>[4x]MASHGKQFTLYTHNSGPNGWKVAIVLEELGLSYEPVFLDLMKGEHKAPEYLKINPNGRVPALIDHKNNNYTVWESNAVTQYLVDKY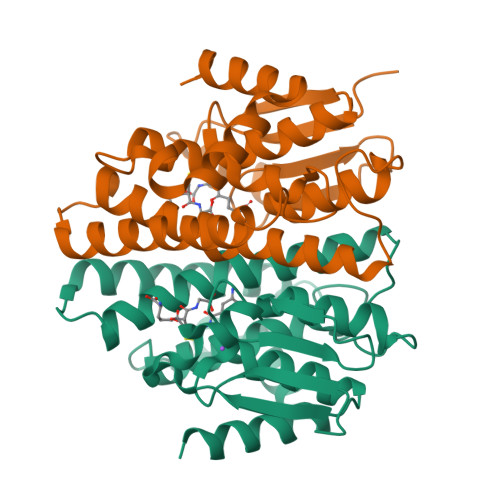DNDRKISVAPGTNEYYTQLQWLYFQASGQGPYYGQAAWFSVYHPEKIPSAIERYRNEIKRVLGVLESTLSKQEWLVGNKATVADFSFLTWNDIAANLLLENFRFEEEFPATAKWNKKLLERPAIAKVWEEKAKAAAH> MNGWNFQELKETPSQTGGPYVHIGLLPK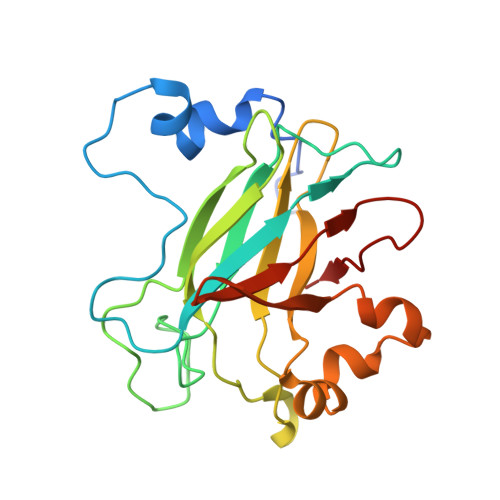QANIEVFEHNLDNNLVQDNTQGQRIRLEGQVFDGLGLPLRDVLIEIWQADTNGVYPSQADTQGKQVDPNFLGWGRTGADFGTGFWSFNTIKPGAVPGRKGSTQAPHISLIIFAHGINIGLHTRVYFDDEAEANAKDPVLNSIEWATRRQTLVAKREERDGEVVYRFDIRIQGENETVFFDI> GPMTSQKLVRLPGLIDVHVHLREPGGTHKEDFASGTAAALAGGITMVCAMPNTRPPIIDGPALALAQKLAEAGARCDFALFLGASSENAGTLGTVAGSAAGLKLYLNETYSELRLDSVVQWMEHFETWPSHLPIVA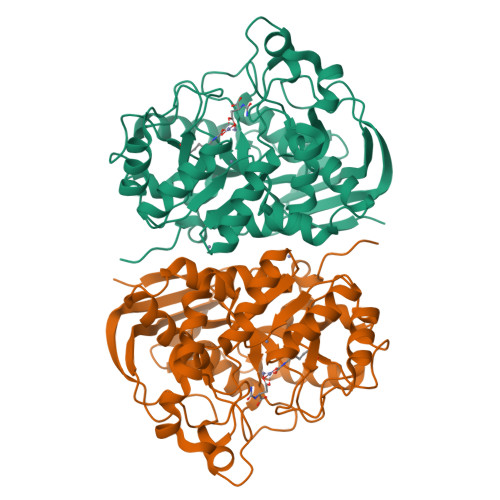HAEQQTVAAVLMVAQLTQRSVHICHVARKEEILLIKAAKARGLPVTCEVAPHHLFLSHDDLERLGPGKGEVRPELGSRQDVEALWENMAVIDCFASDHAPHTLEEKCGSRPPPGFPGLETMLPLLLTAVSEGRLSLDDLLQRLHHNPRRIFHLPPQEDTYVEVDLEHEWTIPSHMPFSKAHWTPFEGQKVKGTVRRVVLRGEVAYIDGQVLVPPGYGQDVRKWPQGAVPQLPPSAPATSEMTTTPERPRRGIPGLPD Dihydrofolate reductase (DHFR) is a critical enzyme in the folate pathway; it is responsible for the NADPH-dependent reduction of dihydrofolate (DHF) to tetrahydrofolate (THF). The folate pathway plays an essential role in cell survival by generating 5,10-methylene tetrahydrofolate as a one-carbon donor for the synthesis of deoxythymidine monophosphate (dTMP), purines, methionine and histidine. Disruption of this pathway leads to the critical deficiency of these key molecules, impaired DNA replication and ultimately cell death. Designing antifolate compounds that inhibit MtbDHFR enzyme activity and also the growth of live Mtb is a promising strategy for TB drug discovery and development.

In order to investigate the molecular interactions between MtbDHFR and the PLAs, MtbDHFR was crystallized bound to NADPH and an earlier PLA-COOH compound, UCP1106. The crystals diffracted to 1.8 Å resolution and belong to the P1 space group. The complex crystallized with four molecules in the asymmetric unit, providing several independent assessments of the PLA interactions with the enzyme. It is clear that there are several strong ionic and hydrogen bonds between the inhibitor and enzyme that provide a great deal of affinity for the inhibitor. For example, the diaminopyrimidine ring hydrogen bonds with Asp 27 and a hydrogen bond with Ile 94 in the active site. The carboxylate of UCP1106 forms an ionic interaction with Arg 60. Several van der Waals interactions are also important for binding: Ile 20, Phe 31 and Ile 94 form van der Waals interactions with the diaminopyrimidine ring and the propargyl linker; Leu 50, Pro 51 and Leu 57 form van der Waals interactions with the B and C phenyl rings. The 2’-methoxy on the B-phenyl ring of UCP1106 does not appear to have optimized interactions with neighboring residues, yet the 3’-methoxy on UCP1172 and UCP1175 would be positioned to interact much more favorably with Pro 51. Although there is a notable difference with Gln 28 (Mt):Phe 31 (h), the active site residues are largely conserved in identity, conformation and position. Despite the similarity, some of the lead compounds including UCP1106, UCP1164 and UCP1172 show selectivity toward MtbDHFR (5.0, 17.6, and 5.7 fold, respectively), suggesting that the small differences that do exist can be further exploited for selectivity design.

>[4x]MVGLIWAQATSGVIGRGGDIPWRLPEDQAHFREITMGHTIVMGRRTWDSLPAKVRPLPGRRNVVLSRQADFMASGAEVVGSLEEALTSPETWVIGGGQVYALALPYATRCEVTEVDIGLPREAGDALAPVLDETWRGETGEWRFSRSGLRYRLYSYHRS>[4x]GITGTWYNQLGSTFIVTAGADGALT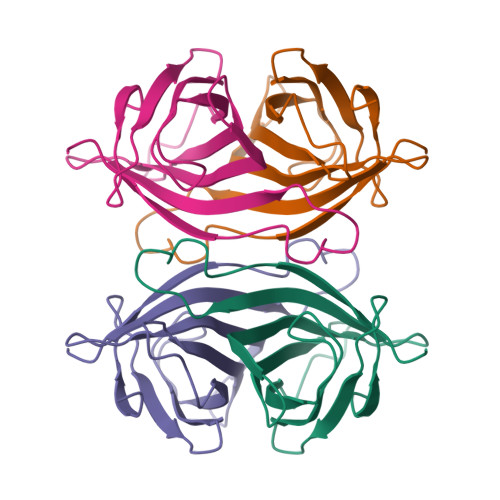GTYESAVGNAESRYVLTGRYDSAPATDGSGTALGWTVAWKNNYRNAHSATTWSGQYVGGAEARINTQWLLTSGTTEANAWKSTLVGHDTFTKVK>[3x]MVIDSKQDLPQYTKDSGSESDSDSSNNFIVESPSIPSSKSATVVLNSEEYEDDEGDDLNGLDAELIDNITYEGDEDETMFVGLKEKQKLHLSGVFRLQVVKGGIVYNNVHYNASREILTFWHPLSQSIPTIDFSHFAGWQDTFFMPRNNRFKIRDEEFKSFPCVLRVFNSNHTGLLEAGHLYRDVNYLWKPKEPYFPLNERTTYHLLHESDRIQSLSVPGYWSTPLEKLYLSHKNAAYDTRIMVIGGKNSGKSTFLRLLLEKFTQDIRDSTTSQEELVYLDLDPGQPEYSLPDSISLNKILSSPISLGQHLCQGSNFQTLLQFYAGSSSPQDEPTSYLNCADKLIDHLEEQAFFGTSLLNLPGWIKGFGMQILNHIIRKYKPTHLLFLETANSKRHLDELTIPQSFSTSLRDAYAPEVVRVPAHSLNHTLSSRFHASQLRTFKILALFHKITQFDYDFAPLLKSAPLQISYGKGKSGIKGIQFPMEFQDLNPQDIKSALEGTVIGIYTYSGEDSLEVKSLNTFPILQSCTSSSKNFITLGLIHSIDTSQQIMNIYVPPCHTQILDKQPEDAQWIIVRNKTETPFCDFLPSPRTITWDDNIQIPFATFERRKKLEHVWKVRKNVMRRGQFMKR;>MIPPRIVPWRDFAELEELKLWFYPKSKGTIEDKRQRAVQRVQSYRLKGSQYLPHVVDSTAQITCAVLLDEKEACLGVHQDSIPIRLSYVMALIRFVNGLLDPTQQSQFAIPLHTLAAKIGLPSWFVDLRHWGTHERDLPGLEMLRWAANEALSWLYDHYWNDEELEDDRDDDDDDDDTGYGYRRNDKLEKYMESLTKTLDKWKRLRNEFLEYKWVW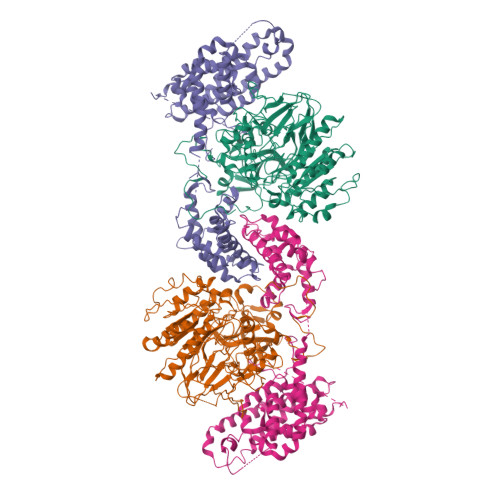ENANDSLITSSNFSGDNLVNYDAEKRKSSHASSSETMIRENLRQWQELWKLSIYHNVVLEKFFNNYDPLLLKVLMLNLNNFDWKVIEWVARNYRTQQDDSNITTILKRKFNAWKELQKRLLDVIINNLNNKNFKNKWQNWEKLIDENASYLILYFCQSMLAKLETEKITGNSWRNKKRRKQIDSTVEIEAKLKENIDNLSLRFNEGEIKLYDFIPAEKDSVPLKKEVSPALKADTNDILGDLASLKQRMSSFGTVGKKNKQEENRATPVKNWSRVQNWKPKPFGVL[3x]> MRGSHHHHHHGLVPRGSMIRTMLQGKLHRVKVTHADLHYEG;> MK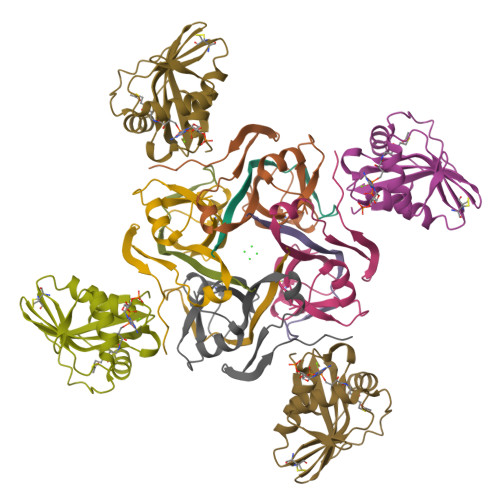LTIIRLEKFSDQDRIDLQKIWPEYSPSSLQVDDNHRIYAARFNERLLAAVRVTLSGTEGALDSLRVREVTRRRGVGQYLLEEVLRNNPGVSCWWMADAGVEDRGVMTAFMQALGFTAQQGGWEKCSGLEHHHHHH;> SCAIDQDFLDAAGILENEAIDIWNVTNGKRFSVYAIAAERGSRIISVNGAAAHCASVGDIVIIASFVTMPDEEARTWRPNVAYFEGDNEMKRTAKAIPVQVA>[6x]GSHMNPLASLTTDKNDLYINWLKSLSFFQTNSSCAEALVKVIPHYHNKLIDFSQVLQLVFSASEKFPIQENQPLPEQLMFLSNLEKQTPFAKAVGSSIYKLVTGKNLSLD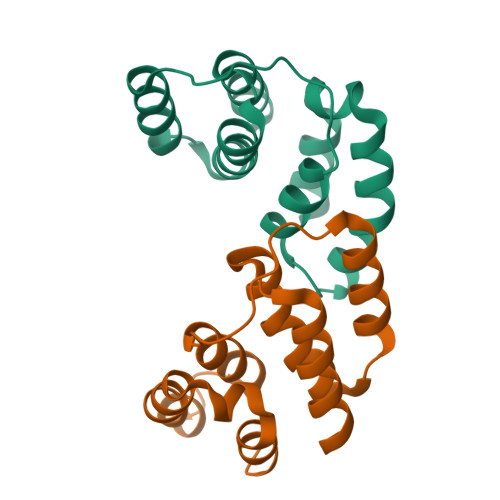FASQILKEASILEH> MVQSSSNEGAGEKHIHFLFNVSTNSLDPHVDMTYIPVRAGITETLVRVDEENVTIAPWLAESWDSTDGQHWTIKLREDVTFQNGKEMDAEAVKASLERALDESVAIENALKIDEIEADGYTLHITTKEPFPEFISELVNPNVSIIDVTEEDFTNHPVGTGPFALESFTPGSKLELVRYDEYWDGASKLDSVTFSFNEDASARSLALESGQADIVYRPEVESIETLQANEGIMVEATETFRTHNLTMNLDRDSLKDVNVRRAVDVLLDRQEIVD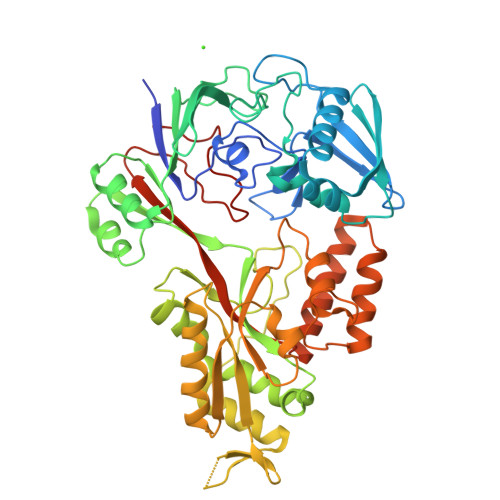TIMLGYAEVADGPFIPTLPFAPSYEKKETGTDIAIQYLEEAGYTLENGQMQKDGEPLHFTVLTYGSRAELPLIAQVFQSNAKQIGIEVEIRQIEVPEEYMASNRDWDLITYSNVTSPRGDAGYYLNATYHPTGALNFSSVNDPELTGIIDELNRTVDQDVRAKLTEQAAAYIDEQKIHSFLIHPSAVVAYDENKVKNWVTTRSEYYMITNQLDVNAENLYFQS> EFPHNAIEPCVICQTRPKNGCIVHGKTGHLMACFTCAKKLKKRN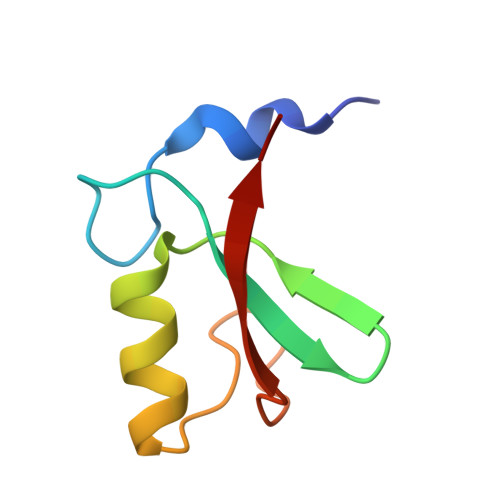KPCPVCRQPIQMIVLTYFP>[2x]MDGIAELTGARVEDLAGMDVFQGCPAEGLVSLAASVQPLRAAAGQVLLRQGEPAVSFLLISSGSAEVSHVGDDGVAIIARALPGMIVGEIALLRDSPRSATVTTIEPLTGWTGGRGAFATMVHIPGVGERLLRTARQRLAAFVSPIPVRLADGTQLMLRPVL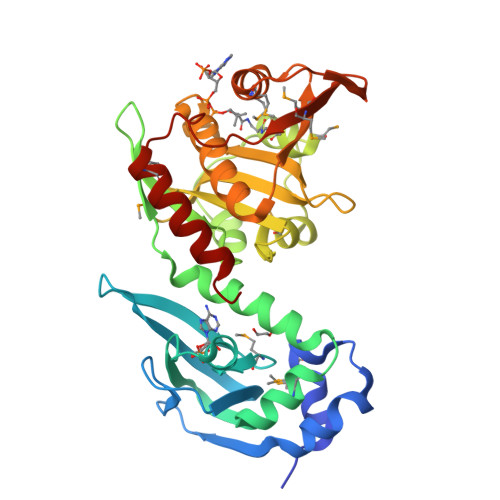PGDRERTVHGHIQFSGETLYRRFMSARVPSPALMHYLSEVDYVDHFVWVVTDGSDPVADARFVRDETDPTVAEIAFTVADAYQGRGIGSFLIGALSVAARVDGVERFAARMLSDNVPMRTIMDRYGAVWQREDVGVITTMIDVPGPGELSLGREMVDQINRVARQVIEAVG>MAAGVAAWLPFARAAAIGWMPVASGPMPAPPRQERKRTQDALIVLNVSGTRFQTWQDTLERYPDTLLGSSERDFFYHPETQQYFFDRDPDIFRHILNFYRTGKLHYPRHECISAYDEELAFFGLIPEIIGDCCYEEYKDRRRENAERLQDDADTDTAGESALPTMTARQRVWRAFENPHTSTMALVFYYVTGFFIAVSVIANVVETVPCGSSPGHIKELPCGERYAVAFFCLDTACVMIFTVEYLLRLAAAPSRYRFVRSVMSIIDVVAILPYYIGLVMTDNEDVSGAFVTLRVFRVFRIFKFSRHSQGLRILGYTLKSCASELGFLLFSLTMAIIIFATVMFYAEKGSSASKFTSIPAAFWYTIVTMTTLGYGDMVPKTIAGKIFGSICSLSGVLVIALPVPVIVSNFSRIYHQNQRADKRRAQKKAR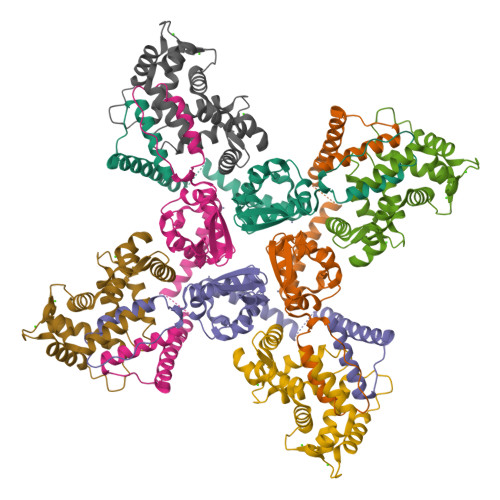LARIRAAKSGSANAYMQSKRNGLLSNQLQSSEDEQAFVSKSGSSFETQHHHLLHCLEKTTNHEFVDEQVFEESCMEVATVNRPSSHSPSLSSQQG[4x];>MRGQGRKESLSDSRDLDGSYDQLTGHPPGPTKKALKQRFLKLLPCCGPQALPSVSENSVDDEFELSTVCHRPEGLEQLQEQTKFTRKELQVLYRGFKNECPSGIVNEENFKQIYSQFFPQGDSSTYATFLFNAFDTNHDGSVSFEDFVAGLSVILRGTVDDRLNWAFNLYDLNKDGCITKEEMLDIMKSIYDMMGKYTYPALREEAPREHVESFFQKMDRNKDGVVTIEEFIESCQKDENIMRSMQLFDNVI[4x]>[2x]QRSYERDFPHHDRICIVKTHGTRQSQE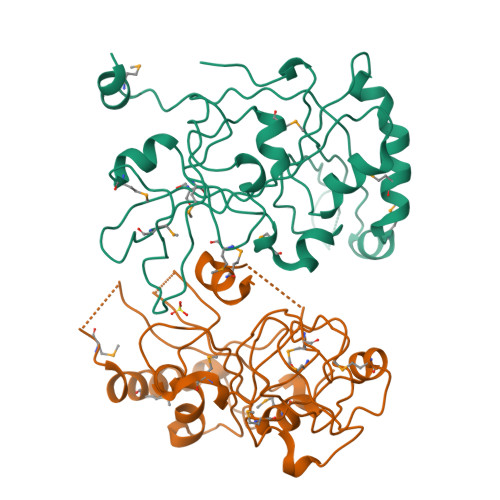GDKPEELDFSQVSGGVAPAIQEEIPGVELATRTTLYGTSKMILEDNKTYETKTLLAEPAFLDMFGVELIAGVRDSALRDNMTCLISESLARKMGGDVLGKRLRPAESKSDRAITIGGVFEDLPHNSSIQADMLLPITWMPAESLNNWIGNDRYIAYVRLRPGVSPESLDEALLEMQKRHQDMEVFRKAGVELHYSLTPFNRLRLEDPTLVNMLRIQQ(4R,6R,7S)-2-(2-CYCLOPROPYLETHYL)-4,6,7-TRIHYDROXY-4,5,6,7-TETRAHYDRO-1-BENZOTHIOPHENE-4-CARBOXYLIC ACID | C14 H18 O5 S | 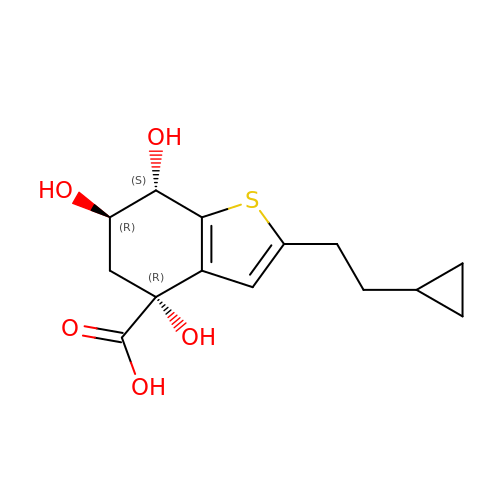ZGKGERUMGXJOHU-UHIISALHSA-N> MFKIGSVLKQIRQELNYHQIDLYSGIMSKSVYIKVEADSRPISVEELSKFSERLGVNFFEILNRAGMNTKSVNETGKEKLLISKIFTNPDLFDKNFQRIEPKRLTSLQYFSIYLGYISIAHHYN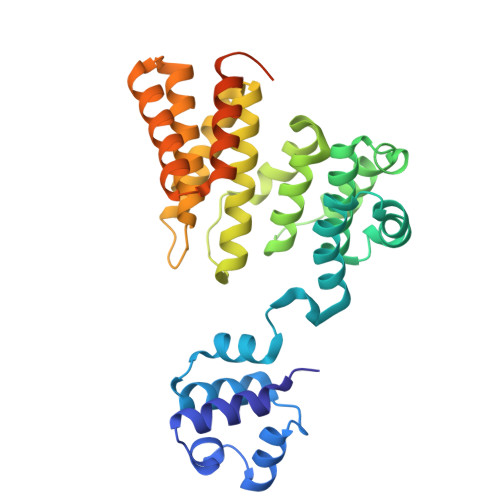IEVPTFNKTITSDLKHLYDKRTTFFGIDYEIVSNLLNVLPYEEVSSIIKPMYPIVDSFGKDYDLTIQTVLKNALTISIMNRNLKEAQYYINQFEHLKTIKNISINGYYDLEINYLKQIYQFLTDKNIDSYLNAVNIINIFKIIGKEDIHRSLVEELTKISAKEKFTPPKEVTMYYENYVAIENNPIPEIKEQS>MEPFRIVIPQADLDDLHRRLDATRWPSEIPGTGWSRGVPLDYLKELVGYWRDGYDWRAAEDRLNTVPQFTTEIDGTNVHFMHIRSAEPDALPMIITHGWPGSVAEFLDVIDPLTNPRAHGGDPADAFHLVIPS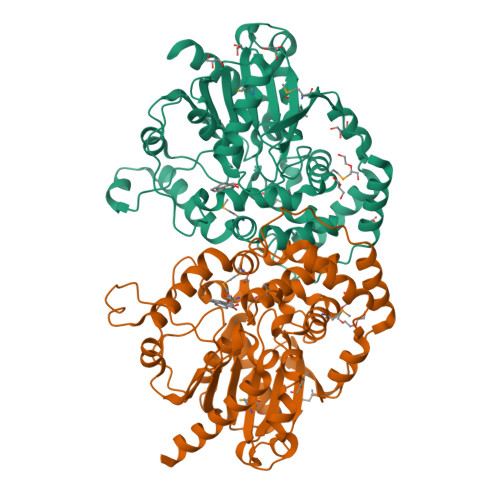LPGFGFSGPTPEPGWNLPRVASAWAELMRRLGYSRYAVQGGDLGAWTSLTLSGVDHEHVVGTHVNFLITPPSGDPADLAGLGEQDLARLQLLAEFGAEGSGYMKIQSTRPQTLSYSLTDSPVGQLAWVVEKFMEWGDTDKSPEDAVDRDRLLTNVMIYWLTATAGSSAHFYYEISDVLPTAPTPPPPAPPLPTPLGVAVYPADSAKPVRRFAERAFPNIVHWAELERGGHFAALEQPGLFVSDLRAFARALRTSHHHHHH[5x]> MHRFRVCALGAAFCVARRWRSGGGPGDRRVRTDWYRCYPSLMEEKDRDMYHCYYPYLFDHGDKMSLYPKIPDNPREWQVEQLQTTYDAIREDKYDAFVRLRAKFPELYQDTYAWDNPPPFGEFNMFYSVRFGMIGVKAFTCKDYDDLGNQFDCTAFWFPDNQIVKHSTRNGDVGTDKVYVGAMNVPVEFHKPHVAAFYKAAGVPVKHVSAGFPVTPDAYAPVGTKLDVRHFKPGQEVTITFQNTDYGYQGVMFRHGFDGGYVWLGDSKWQRRPGCMGAEGQKRIYPGHRMAGQTGASAETYDGVPVWRIDYKNSLIYLPTLIDADVGTYVKFRDTINTKGYTLWNEHRGTPPFPTFIPSEEEDLSKLATDEGQLTSPPLYMYFRDEFAAAQLVTQADVEDAKSAKPATAAPKKKVYDLKKYTEARKKYRKNLQKARKYKLMGVRTRAHEKQQEARRAKILKYKRVKT;> MLRLTQAVLRVQSHQKKRAQHPNAGTRFGRVYNRGFVRYGFGGFGMSVYSSKKDRTFKVMPVPPPPPATTAVEQRDDFADNRGLSATTRTLSPTFRMFALEDGGVLVSHPSHAQIMRWNQRVHTEEGKAANSTVMDEYVNSRIQAIIADNTIENTSLSQWRKAHMWNVIKSHGKLQRRWGTPDFVMGARSTLYNN;> MSRNGELCLQRIIVSYSPNKGNPAMRQFMATHLPEFHRQYPQVKIDIRPRQWPESSITGIYRDGSEKAYSIRFLSSMGINVRFHRLVNEGNDYNHSFSASHLHLQRRSVQGTWNPYLWNYEGTRARHKPPAQWSRKLTEKEWDYYVQQYGAQMKAEEDTIADRVRRYTDIPEASTEEVNQRWKEHVMPRLQTDLEYNLSHWKKQHRTGAGRPAPPTLNEYSLFSVPDHSSLGQDAIDMLRRREAQREEDWWRERKGQLKPPE;> MRYCRPSRPLVLARASSVLSSSRTFHSQHRTPIIPQVHVHDEPTAQRIHVGYYLHRHPVVKHSPHPLETEMGYLLEREQQRYSRHESAESATAFFASRGQTIDILGRTDPNQIKGNFFGLELYQDAMKVVMQRYTPEKRLTSADLWQPNALGDAPPPRHTLHRKLDDFLYLIVQEGATGKWTIPHTARKDDESLRMTADRAISSQNSEGLDCYVWSNAPQATVFLKDDNTRLFIYAATYLAGRPQFASFEPKPKDHAWVTRHELLQYSDTFKSAELLKALLDISADGTFEA;> MQPRRMAGHFNPTPQANSLAATHYAHTPELRHMADGAAMSLSGQRIPLLKPTLSKWSRQLRSDIYDELLKLPLRYALHDFRTLQAHIHAVPATATNASCTAAAGERLPPGVYHASSGLSSASPDAPAYYAVAGRDSAVGYAPPLGPADPVDVIPFFVHRSSNGHLPGKVYSMNAKTLMPAFYMRIQNIEGDMFRFEEELMKIFPTKKIFVRSHSVYVYNVNLDGRAVLHHWLLGLGF;> MTAPASHYTFANLKKLGLCAPQVALSRQPRLRPHVGHLNGLVYPLPYYAMWRGNHDKYTYNQATPARWGEGNTNTMYHQHYAHAKCPTDYGRGGREFQFLSVKRGKLKRKPLPTVQYVDPNSKPQWVFKSWHNPLSAPSMWEREVQYPEHTPAHTGAKRPLAVVAPKTSHKHLFLMHMEKVTVTVSPLLFGYGHTLQKAALDFYRRGLSARSPFPSDKMFLYYSIDHITPKIEVTWLDGSVYVPPLIEGVKAQDLIQMVMEQAWLAADRMSAEGRVLNPIAIDDYKWEQLIAFKQKRAKGAEAAKGGAKKK;> MLRRSPVPRRYRTAWRELLHPLPVWARRQQWLKRDTVEMNEAILREPYYRIKTFAQPAAFVSPRVSESAAHEPDTQQSSRYGVDRQLRGPRRAVSPERLQELREQLQFVGSIGPKVPPAAGAGTAYQDEYGTRLRPRYPQSWDTVPPHQPSRSEI;> MAFRGSSARLAATPGVGIAPETTPVKYVPEMLNIQNAKWWNGRGKPVYRSTYNEKSWLEKARWGAFTKGSRPVMRQRYSAAALKEALEMVPEGFETCDVPRPPQRIRAQSEGVVGRWYTNYWTLHSVRYQCQLAGVEWQFGERQRPRTNYDEPHMYTDFEETKAIRDYRSRWINVNRSLVGMSRRMKESEEEARYLHFKKVQDTFWSNRKVLVNRIKSMHNQGTLQSAKDLPIKTINIKAFLAE;> MHLHISSIPHRNSNNSKGGVLDATGPMLSAKRGALLLQAYHRPGEVISYKAGDYHLVPKKFTVGKRIAVRSYLDRNRTELSDRTFMPQKNWFRPYDLQDGCFDRDHERLSYRFYNLETKVIWKAFDTPELIGMLLHDETVKGNSGMYAPDMLDAALHYTREARYWRCIGITKPFYDRNTLRAHCWEDNGLQVGTLVMSQAMRHALMDLERAVRRKELGLEPNYLWDRWGPIGFIDGARADYLPRFEHNPYVDPDGVDVTEIDVLPFNTHEQIRERYRDFIEPDTAPFEEVFRSPSHGSLTTLADIPNASVVALYKDLKLKAGTPVAGDAVELAPADVRTLFYLSANPEWRAVADGKASWEEVVDAMQPVQAELDEKIDAARLLQNTRHNAERVRAFFEEKCGFHDFMYTPDKTITAAVLCYLTELRRICTETAWGAALAKCLTDMERVQGMGRDAFLVYRHIEDAILDKKRRLWAGRFAGESHEESTLDYLLENFGRRAERPRNVGTTGVEFDREQEPIGRQVQRRVLDSDKANKLAEIRRSRGKMWSKKRSVFDALHEKQLQNFNYGVH;> MPAYSEVKGTCGTPVLDQLIGYYVNIQSRKMYYKDFLRIEHQAVRWAFADIRKNSEALAHGLLQTGVRPGDRVLAIQPCNCETFVLQLSCAKIGALLCIVPQDTISADKLRFYLNEFQPRHLVAREWINVPEMKQGELVERNMHFWDTIYNVIPELGLSYPGQKFQWVHSQEFYYLKKIIITDHNMNLLGVTPMRKMLVWGPFSYYEQRLRRLSALLHPDDPVLALEDPNPAMEDKLHITYSHRNCVNAGFLFGQLMQLKAETRFGVMPNHHTDPIGAIIAPYAALTSGAVLVHIHSDMFTDDHAINGIEKLCVEEVETLVGRKADFDLILKHAGNFDADQFEHLRSVVIFEDGIEAPVSEEYLNKLSKALSLDDVYVFRGPIEASYMLTWRTLKKGSQGMVPHVEAKVVGDRGTSDAKVLVAGTRGNLRLKGPHVTAGYYNNAGLMTELIDEHGFASTSREAMIDGKDNITLMSAQTY;> MCTRVFDVSQRFILLVSLPPLSLSLRPSCCSRKAATRRRRSTASVLLATDALSLFVRTHYPSPLLFLLLPNFPLPIHSPRKQMRAAVGAVLQPSSSVGALRCQARFITRLYTSYFKGELFPNQLARPLERLPRGVSLAAARKGQQAAAPSSSGSGNPATTASLDVVTWGDVDSTDLVHANEQSRAVAPQAGLAPRRPYVPLGEVAKLELQGDYLTEGGLHQEALEYYGVVAKAYELAYPKDHPQVAGIRLKLAGAFRRTGRLTSSKANCEAVLQMLDSAVQPPLELIVEALFELGLTSEAMSDAAAGTVFEEAVALVDMFHNSGQSHKMLRLLPRLGRRFNLNFEEKFVYFSPFDYDRVFALADQCLERAEVFYQARNDRAGVMRVLQQRKELIDKKFFNMRDFAGRIHTMRGHWKRRAQVLTNAPTPDELLRYSPTIHQVYRDFKYELNAPIGREKEVQPGVNRVVHDMGNPYRRSGVRSQRMFRDAEKNFEKYIRADAFEA;> MPTTVLYHGDQLGPRPLVILDHSVARLEQSATAVLDACQEAAKRYEAMLSSLAWDHGAVFVPLQVSIGEINVMEQSCRHVCAVLDAMDVQWSHVLAHSYGALVAARMAASTAYPHRIGSLLLLDTPLVTEQLVRNTKQREEIAKAKKDVNVPPAELSFAIESLRSALETTLPYPAAVDKSLYEDHLFSSASVFREKGLVRDEHRYVPVRHLAQVHHPLQLLVPVKQPITDVAIHREFFGLRRPAVIKTADNHEDLFSAKCADEVADVVRAWMQRFEPDVVMKRRFEKAAKEMVQLMGSSASFGEKGGGNIEKSEKKEKRKGRQ;> MLSSAHRAAFARPTATLWASARSFGAGPTRLLLGLEQVQDVPTSTDRKPTGMHRGPGKRQTAPKEAAQYQFIKKWDLQMRETWDELEPFKGLPKPKVQFGNEAAEVIWPYALLLENVIKVHPYTKSIYVYYSQRQSTPLGELAARVAKRVSQAYLIPITFHNSHVYVEAEMLLEYSETPWVVVHCLDGTHKLIPVKPQAGQTVKEGAEEVLNGIVSACNEIGSAVKNPKEVMRLLSERPLQNQYVRVNYQWYGDTPEERMSHLVKWDYEPEEVVPQLRNRTQHVLDWMNYDGNLPTHNSVRVNIHREAARMRKPNVSAGPKTFFNSSGSRANARTARFDNSRSSQS;> MLRRTEIALKKGWTHNPGHTRRGGKNLAWRPKISDAKLSQFVPLALVHPRRHPNNWQERQFNALGYTKWPKDIGFYNAGDNFEVTPEAAWRLYVHARDEPYWGKLHCEKTIITLLPVVEKAPKENMERVLDVFRHYLKRYGADHYIYNAVMQAAAFAKNYEQAEQLFKEMETLGLEPNAQSYVNMMLAAKLCGLPPEKSEAYFKRAVKDGAMQSVMRMDTEFRMWMDQLDRLGSFTASSGYLSVNEEGAKPMPRDMWAIWGWHRSESKFISRRDLIMQQVRARVHSGKELVGTVYTKTRRQPWAKFNGMLRHDYNGPSYRAPTIFPDAPEYTNEAGHKAF;> MLQCTALVLKSQHKNVLRKGRPHMQKYKELNRWQREAQGITKWEQGHSHRPQPYVERFNPEGAGLTRGTSAYAWKWWHTQYPWLPNVAPADYVPPSPRGIRPAAWDDEFADVVLSMSDEEIQSYLLDKLTEVIFAETQRDGYELRRLDFEGKPLTELPERRIIENFVFEEETLRERVLDRVVEGVFRLVPTSTDRLELKSVANIIDFVLTHVTVARKPLQHEIPEAARTVMRSHPLQPQLGFVHALPTDNRDAVVQEWERMHHLDWQFGKAVYEPRSAENERGNLTWLREVRHHEAREAFQADVDSGEARRRHMAKIKAAAQVPHTGTTSQ;> MLRTTHVSWASTAKGYMNRVMVYAHRRRKARYLAPKNAHVRSPLAHKMPEEYGNTWDPRSGVEWHNRMRNRNHYRHWPWARWTDDPVRFHQDSVCHRTVSALSTVANNGAPEWDYYAEVGQAYETPSHFPLSYTAPFIYQYTAQCWSREDLQSYLERIEQSSGLRTIADAASRREALYTWWHNAGMNVIPLGVLQHLELVSRDIVAQNARKSYRIEQHERGILRTPEMERYYALPHLRGPSMPVQLAQPSGKYPSGKFTQMMEDVAIHPLQKPDARYKHNMYPA;> MQRCLARLFQAGVHTPHGSRYNAARMKNWPVQEVPQNFNFTNEQRFKAKAVPRDTGKIPRDFLLSVLYRNQPCEVASLWEHCLHDPQIVLDSKRHLREVLQQARAEGFVSFEKDAVTDRWVCHLTRERFEEVRALVGARAEAQDLYSGLRGASATETSAYSESFREMNEDTKREHFRLLSEQVADTTTHLRKFQRMEMDYLPYTDLNGKVNFMWWYEMSDTRDATALPEAAAEGSPKLSE;> MLYGGSRVQYLVQPPFTLHKIRSENLPPPSLYAERHDLGLEMQLPRDMHVYNSINMAIQRQVGGDSSTLDGEQQQLQGGHADGFDMGAFFTEQHHPERHHNSSLPYAKHDTNNVLAMRLFPVNVGVRARTEAIRIRTDDCLQRLRDADLCAKMRLPLEHPLPLSRRSQYAAIHRVRQERCYDAPTEAAGERAAAAAEEASRTAHLRGAAAHPPPSELSIVTRPVDRLGSHSGSSAAACTADADHLSFPVHPFAAAAVSSGCHSARSGSAARLASQRWLPLQTLKPMGHNWSAATRSSGVRGPHMQLMQERLDQKGFGWKRKSRSLWQQDVATAGFRPHRYF;> MLRWSRLLREMAPELQLEYIPIIFTRTILGPQGGFAGEERLIKREVAQKYMSEGNAVTPSAEFHQGVWCYNPDSEQYDRFVERNAEFLDFAARKRQWLDVYWRVNTGYLLFGRQSWGQGWLLNCPLRKKDIAQKLWEQYKVRVDPRLIEFREKDRRTGIQDLGHNWCWLYLPGAEELAIDREVYDNKRVKVRMHIRKMSSYGALY;> MRRLPLFCRRPSRCCGATASGSGSSSAAVLAASAAPSVLVLAARGIATSGRVTNEDRRWWLVHLECAPDVTPGTFVSWLDCCGTHTTKKLIERNIWTIEQVAELDSDRVDELKYKEGCLKMDVVWEHARTIITPLKQREVSGGVESQLQSRILELRKKRELERQRELLARERATVSDKREETLRRLRESVAAKKAALRKKLDEQHGEATPAASESASTEAHRGTAEAAVEDEAVGNIVDRMSGGNPPRA;> MRPSALCLGGFTMKYKRGTGLWDEDHVNDFDANKYLSARSTMRWYYGMERLQTRNNMNARRATQSYNNNMGLHHSGRGAFERELERRGIQVDKYPLTTTTGAARVAEMVLLRRQELEAHAKKAMESQRQARRRDAPSEWYDETEGPLNPRFLASMQSNYTQVITELPSSPVTGRRELPGASFA;> MMLQHTSLLCRKALQSYPVPPRARNYERRWSSSRTNPYNRMFWRTVLNEDFARPSFWVSDFRHKYLAKHGMDYQGRVPASPAPGMYQGFSDVHKILANHPKPQRESRHLPVMPMTPRVVFEHAQEKRIDYAKKMHRDRRLVEQLRTHEFWGWYMKLQRVRGRWCKEHGVSSRGVYGPAVDAAELWG;> MFQRTCTPRLLACTSALLKRSGKPSDLPDYKQVYLPYDTAPTKTELDRERRKFMHAYSGRMEHRKMVEVKDVPQNMYTYGKEGMSIPISIFKDQADPVIGPEWTYPGIFENKIVAQHWYMEELFDREKSNTFESPWQRQVLDNQVKRRLGKVAWRMSMLNIKTIDIFHKERGASKRPGAGDTKAPATPAGKK;> MSSGAVGRGSFHSVVAGANPRRIPTYYNSAYELIQLHRAHREVTRNFLVRDKVFDNKFPGCSLANGLFKMVPNKRGNFHTRELTESIRHRTIWGQRIQQQRTINAAILEDATKVLSPAQMEDRFSYRTPDAAAYFSPQEYTAANNWPNYWQHPTEKHVVPKPRWRREPELGGITRVRDAVATPIADY;> MYFYRRIPSLASKMNHMRQFSLPRSSAAIIMAASTAALAVPCRAMHGKPASGHKVRTQHSRRWWMQSKAHHLTAVPHEEARSRPHFPAYTEDVDQPMVVPDGVCCFNCDKPIDGDDINSYVWVPSGNARVPTTQGYFFHVKCFKCWNCKYRIIHNQFYSKDSRAWCLSCALGRDIRVPTRRWHTSYVNTHRTGSRLTGQFFPRHRHQMEFLFSPKE;> MLRIGRTLLAEVTTINSTTASVSGRLIRIRKKSKWIDRRSTRVPHNGKDIWYFGDQPSCALCHIRFRYKQDYEAHKESELHVNRLRWVETMNWWRETGEPAYLKASNEQWEWFEQHVLPTKAQEMGCTLDEARRVYRQAIMTETPTWHRPLQCPTVKQEVQEPRDQRWPASPKW;> MLRFTQVIRKNPVVFKQGQGMFSHQLKRILNKKSLHKYNWDPLHMYDPRKLVHANRYVDHDTYEEKYDPHWEHNAHLVPDQQFYNIPVPKEYKDAYWWRDLQARRVQCPTEWVHFRMHTKDKLKYDFQDLAFRKKFEYSYEDVVANAKDMCS;> MYDSRSSGVHDVAPRDGVDFMYEGPQQVLPGAHPLPLFHPDNSVTRPPVSPYLPSPQRPHPYFTTELPELPHFQTTRPIVYTVGTMKQRIVAPVFDLANNVTHTRELDPFIFGFYPETEEMAKNLSYWLVRCQNFSSKWDYENREIWRKAKKNWPNTGMGMARVGDRKNHAHPWGAHSKPVKPWNLLMPTMDVKTWSKSNRMLVTLKMLQGKLQIVERLTLPEPTQEAYLQLCRTMGWDVRHKGGGALFMDGGSRLTPSSEYDRAFFFGSFFNGRNKLVRPTLLCDEPYDYNRTSSKARTKGPKGQKNPIPINRFNAYDALTHDTLIITEGALLQLEDEMYTHKLAMLPPHIRAQLPERGFLDSEVLGDVPPALQTVQMEAAARTEEAEQAMYAPYYDNPYHPWQDEGEASYAVDAVEGTVQRYIKSRKTSWAMLS;> MAQWIPKTAWKVSNLNKRYGAPYVAKGYASLDPRCSLDAYSSFQQTVTSADMKKALLSIDSTSSGALVIDVRSEPERRLRPLLSPAIVALHPHDILSGAACPILPSNKERAEMFVVASEAQRAVNACTALRRWGFSRVTAVSVDAVSEAIAAVQKPADAATSSSTKS;> MLHRSCVLVDSFKEHYHRVHLPRRLALQRYIKREEARLSRHKGKAVAAAAAAGVQPGEVAYKYNRWWVSNDHEFVHQFAFVEDPDVTREKRNTLPLVTKENIWKEPQQTFFLPFAPFVRVVDYAKDPDTKFLKPVNIPRWKDYMQRTKPIVPRTWY;> MNDIYARRLAQTSMFHQLMRSHGTLWAATQVTKEKLNLAFVKEEMMRVNGRRAMPLLIGAAANENLNDTHFTHLTEHCAWTESARAFAVQRQTPLTQHIASMGRMAETITQAKTASTSQLLFNEHLARIDGISEFEEEPFVDDEDDS;> MSNRFFQKFYLRCGNCSAIQRSAQGYQPIANPILFKSDEHCRNYHDEQRRAAGYSGMVVTCRCHRCERVHSNWKVLDAQQFLDAKLRMTPEERAQRLWVSKS;> MLGGLRPLAAATRRTVGGALVSPALITPSRALSVRTEDFFSKEAVSHARRVSWAPHTTEKKVGAFAKLSRSNFNDPLPVSFQSEPYFEEEIEAYRAHHRPDVYVYKYNVSPTHLSLRE;> MRRTVRALYNSFERGWKDKTVHPLDRRGRFNLDEAAAELQLDEAYVASLYKPLHYTYSMKGQRYPAEQGRTSRPGSLAASRDRMFPLYRRNYKLNRELRVLDHRRISTD;> MLARYLDPSVHPLRVGQVVAYDYLHAAKTWQWTLGTVREIKDYTAVVQQWGLHTGDIDTLRSILLKEVDTENGRMKNYHDMLAIAREKLASIRRSNEDRVSHVRGHFDKAREKVELIDEVDLRKVTAQAAPSPVAVAVLKAVWAVAKCDPTAVEFYEWADVQLEYRKPAALDEIAKTDVLAKLYPSAESLQQSLEQDPKLNYKAAARDSPVVASLHAWVITALAYQQAYNLLAHDKRIQEQNDAIAAAIAGMKACRAKIAKLKDELSSKDTAALPGQVTSFTRTSVLVTIPLSAVISPVNVDTDVKRCVLTKDEVEQIPIDAKITRYAQKQKLAITGSHLLDQYAAATTTHIYVTELEDRLFFFQHYMASALRDAQTAAVDAHQRLAVSLHELEAFRQKRHDAKKARAAEPELADADGVEPSSGPTSSRSPTGRAAPRGQSAAPRGTASQQHKLLGPAYQSIDPATIANEPLYAVTIEEYKAKDAAGERAMDEAERMADEVQRLAVELEDAKAAADKLAEELAAKDEELAAHRQKRHDAQQARASDPALAAADAVAPRSGKGAASPHVGAVQRQAVDPATVPVAPAVIAEEPLYVATAEELQHVRDFADQLAEELEAFRQKRHDAKKARAAEPELADADGVEPSSGPTSSRSPTGRAAPRGQSAAPRGTASQQHKLLGPAYQSIDPATIANEPLYAVTIEEYKAKDAAGERAMDEAERMADEVQRLAVELEDAKAAADKLAEELAAKDEELAAHRQKRHDAQQARASDPALAAADAVAPRSGKGAASPHVGAVQRQAVDPATVPVAPAVIAEEPLYVATAEELQHVRDFADQLAEELEAFRQKRHDAKKARAAEPELADADGVEPSSGPTSSRSPTGRAAPRGQSAAPRGTASQQHKLLGPAYQSIDPATIANEPLYAVTIEEYKAKDAAGERAMDEAERMADEVQRLAVELEDAKAAADKLAEELAAKDEELAAHRQKRHDAQQARASDPALAAADAVAPRSGKGAASPHVGAVQRQAVDPATVPVAPAVIAEEPLYVATAEELQHVRDFADQAAHDAATREAEVAGTVENLRNELDDVREMNAKLEDEVFALKEQLSDAEDAYKKLAGALVVAEDERQELCDDLEAALDELEQKKDEYDELLGNLEEVQGLLEAADVAGRTAVEALEQRNRDMADLQGELANALDASKENENLRALLDAKEREIDRLKEYNSFWTDTVGTGKQKVTHRLTKIFDGDWTRLMRHRPEALKAAFVIDSSNACHVPGDQIFLVSNSFTRRLLTRTDHCPKCDRLSTFRFMSVSGMVGRMPYKPVDTPGPSYATLYWRKQRSGKIASQPLNEVCNKNEF;> MWRLSRVALQSNRAALYMPYTPVATNPVVYFDITAEGDALGRVSVELFRDVVPRTSENFRSLCTGERGYGQCLLYYKGTPFHRIIPGFVMQGGDILTKDGRSNVSVFGYPFPDESFEGKAGKHLPGTVGMAHSGPNQNGSQFFFNLGRNEQLDRKFVVVGQVLGGWEIVNQVVKLCGSRCGTPVSRAWISDCGQSGGYMAEETQEALQGERAQHVIPGKEVLDLIQPRY;> MRVWVLAPHSLPPASFRPIFEARPPSSPTHSFHLLPTPIYLYITCTDAVDLYVCAVTSLLAEWTTTMFARSTIRWAAGAGHAFMDIAIGSQPPHRVTFELFTKRCPIASENFLKLCTGENVLPQVSSIDGIGEPSFRDQFLPQLTYRNTTVHRVCKGYLVQGGDIVSGQGTGQLSIYGESFDAPEEVKASKFDRMGLLGTAVSAPHLNGSQFFILTADKAPHLNGTCICFGRVVDGWTVVKAIEAIPLTAAGEPAERVVVVECGKL;> MASVSPLLMPCRGVKLVNPIGKQGSQHYGLEPKLEAGRDTQLKHTEMYDGYTDDFGVFKEGPPVTLRLEYVRSPDHGYSQHILQKDIWSPFQVGANMMSYTPLYYDWKGFSSRDYFGHRSGTNPGSKVLLGHYRRDEVRSWGYRIMVNHKPQKRIPKWLACVVHIPRKKTFLGFFLYANGAYVAELLTYKQLPRIIYNKAFQGCLPTIGQTVSLTEVTYGKEIHSVEMYPGHGGVICRASGTAAVVLRGSEPNLVPLLLPSKEVRLFDNMCHAVFGRRAGVMYNKQRNFSKRSVEENMPHRPKVHSKTKRVSSHPAGGGNGGSPNLLTPLDWRIHPRNCVKTKYWLSGYILRGRQYNRNQTVADLKSKTYSWANRDPVYR;> MSVFPGLCGDVATTNYRVFLGTLPNLAVEERFLRQVQPVFPWYASRKHVKEQASEFLEIDLASCDPELLLRYTHVYYVRRQLYDELVDRQLTLMETGKAAKVADSALLTCLAQVNAAITPRLQYELHLLQQAKKACRVPRRRELNPDAALEAHDYLCMMRVVEEDVGGIPDAEMQARAYLPREVLEAKVKELAAMIFGDGGSATKGTGAALERKEQKLLQRMIPADYNKVGAVEKLRPVDVTALYRFTGERVCGRPADKPFARALWGHVFRKVGSHPLYLQRASLYWARHSGLDPQSATSAMPADLATAVCVQQALFPALKYRCQYLYTSPDIARQQWRTGHVVPLLRLFPLLGAPAAEDLAAQLVVEGEWAKLGIEADTNLLHDTVLRQLKDMVEQVSALYESDAGAVLKRVEDGAKVLCPSLSERESLTMRGAPEDTSREVSAAAAARVANAAPA;> MLRFFRARLAPTTTDAAAKLPAGNPVNKTWFRHNLIIRRKGSYRSRWGNGTEGYGAGVPLSDQVKLHCVDNTNCKHVRLIAKATAERFAHCRVFPAVAHRVSVQRFKGRGGGGEVSRHRVKPGNIYWVCLFTRRQTNTRMSGLQTNFDRNTCIIMNDQRVPLGTRVMYCAGRHVNHKYHLKAVVLANFFV;> MRRRDWCGVCLPAATLHALARRYSEYRSSYTGARSAPWAAPEAAPAYPSARSPFPLERPRFRKTHIEWMLHHGHGDRYGKYGPSREIADFEYADGTPSSISGKRFALKHHQDHLLVQLIRSAAIVERFEEEELLPRIPGTPEQRSWDPEIPLFLEDVDEFGRPPRPVAGNMVARVIEERFAQESGRTPVNLANKHAGEVLEPNTMFATYDPAAFVSDDIKKDVRRPFWSRRRWALSDNFMVPMSPKPKNTIKDE;> MVLNKWAAVTKSAPPAAGLRPLARTVSPNPKLRPADYKVPYVLRTFIKDRHSSEMQHIENRGMYREELAIERSRFPRMQKTLTIQTDGSLNEREFEFAVPPVVMLFQDRLSAHRQRQVALAKIGKLKRVKSWETSVRGKESLNPVCNALVFPYCVPKKMLVRPRIVDPLSAKSMADNRRSRDDPS;> MRRSAWVFVAPWVPPPRHDVKVTMPPPPGGEVGGSYGVSTGYSDRLARTPYWKRMALSTYALRMKENETRYPMSPHREGEYDLRYTVTAYPDHIKHRPLLEIGEAHQIPTIEIPVIFLVNLWDEERLTWFGRQYETVYVNRNVAREELLPQRYAIYATEEAYKLLGLPVVNHSIHEEIPKTPHAYKKLLEKQSYTEERWKYTIEYLFRKYEADPPELQDKSEDGWDGVEELATSATAGGAGDSLAKRKGPVKQRKARKIKLF;> MFSRGAAATAMAKVSRLVSPRLRIIHRDYLTRRGGRTHQRCSAVAVDYTPTYFATYKSDPGQCPRLIDAEAVHGDEQAFWSARRDFYRGGASRSYYPAWDRQAQALIMLTREVPRIPQEAAFRLFTLGLKMMLLPRLVAGVELMLPSWVTMNAESVLNEGLEGKVAEADGDGKATGAAADAAALPSASSAGANEDSGSANAEKR;> MLRRSAVRYLKARPKTVNIEPGSNRFLDPNVEAKAKDIFAVPEFPNKAVLHNWRFFIKAGKAATGPPVGQEFSKLGLKAMDFAKAFNDRTKPHFKDDIELIVRIQVYFDKSYIFRIEPPPTAWFLLRAIRKKRGETGPVVLRGNYCAYLTLEMCYEIAKMKQMSWGKVEYPPIEVRVRRVVGQARRMGIAIIGIDTVHSSPVKGMTEKQYLEESEKHRKVHMIQYEALKAKELESAPLIERLHRPNMAPLTNTQLEEGLKDANLLNALWKSSHPKSLFTQDTRDREMARRYLNTRGWFKEMTPEEMRVVFLNYRLPKQEDHQRQLNMTNGQAQSQAYWSRDAASPQ;> MSKQWLCREGERWWLLDARGQQLPHVAKIAAQYMTGQHRPDFTPGMMTGDHVVITNIKDAVMTGDNWIRVPITWQTAYPGGKYRVRLSEMYERDPCMVMWWYLKDEVNRHFVRKLKTRTAPLEKAWLYEDSVHPHAEKNPRPLVWTDTATMGWRYKDPTFQRRWSPNQFMS;> MLSISAVQRRYRLFHPVHQTVPFHFNPVQSIFPLIYENNLLAKPRLSWKDYEGRKEFDADHPLPVVGTRLNERTTTHKWSHWDQYINPQITQSWMYLTQTPEYVGPRSGHNVIKMGWMKIGGSWKYSRSYNDARRGFAKGQWQERKMTPRFMLAPRVSAGGPRNRYEGKASFSRLSLSKLLWAVDTGRLNPNETITLYHLRNAKVIADREVVWPGMVLLAGNVERVPYPLHIELQNASAKAIQLLEEAGGSFTNVYMSHEGLYQELHPEEFPTFMEQELPERKGLENFATNSRKRGWLAQWYEDESRYAHPGAGRRTAHYIRPPTDRDFPATIEEYELAKHHQKWHLNQPGSATVLPWHSLNTADMARRSAGRL;> MQSSALRPSSLLRAYHYVHPKTGRPIRQYRKYGDPRFINNEVALIKGLFALITTDFGMVTQSQLENARLAILRRMPRGSFALTMHTDYEEFPVVQKSPESRMGAGKSNIHHFAYKFTTGVPLFEITALSSRRLNQAEAEGIFLAGRSFIPLQTAVVPRGRVDEYHVFK;> MLRWSRLLRGRPPPVMGHAKRMRFAGVDDNPSVTHKPWDTSEPLMADYGWERGKLPKFRARSPFHRQQIARRMVTELIRKDYVIVGGARAPALRILADHVVELAKAGDTDSRQQLAYFLHDPLMVDKAFDEYPRRFRDMNAKYAMMTRLKGRRRSDNVAMYFVEYKNRDMSDNHKGEDYTAGPERFFLPPRIIETEKGIQRPPHMQMAFDRWASKFKTEEFHHWWRLRHAKLRYWGVRNVPHPSDVDPLWTEKEEEEWHNEMLANTSDFEDFDLDDDSYEAAGEGGSQGGSSSLSGIGPEPQKKY;> MGYTRERTNRHFFVSRANAFFSRLPISRIQRALAMEAIKKGSMKPWKHTKEQIIGSPITCNFEYNPRPVRLIGTVMDAHTEETSIKGGLKVYARSEEANMMLWIPAGNPKLKYEVTAAKGSFEHYLDERSKWDEAWLTGRARMK;> MLRSTGVSLYYRATAELDRLRGMLRGRARLERKVGLKRITFLMRTQTRYRVEQKAHWERAIVRKNVDSAAHEHGSGWQHLRNDLARQNLMLLPRTQQQLAQYEPLAFRAVMELCASRVAPPPPPMTAQVPEEAYATRPEDPKVAHPAARRQLEECVERMLCTGRSDVLQREGPRTTQAWMDAWKEYDLGSAAQK;> MLRSANPTIAKALQPLIEGPKFAVVYCGNHQYKVSPGDVIAVQRLRAPIGSQIALKKVLMVGGPRFTAIGRPLLEHVRVTADVEEQKRMRNVVSLFSTPGRRRLRWLDAQHAATILRIREVVYEPTVVGELDKYDGVLLKDFHADRHPNPVFTANDGYDLYYPKDWNKVEEASAFLEMMEAPPTEK;> MPKPAPRYNIGLRPAPKRQNVGGQFLATQKHYARELWYKRQYYSTRPFAIQKHMGSTPRILLDRTLWRSCWLTKSNLPDVNRWEKVVNSQRVTEDRWALVEEDGVMYQVNWKMYCERLETELQKAQDQLPQYSFMMKAVPSAWKKLDIELSVLRGLSVREAMAQCKLSPRKGHMAVFRALEVAQQGAEGKGLDKEHLRIAYITCMPGPTDKQVDIRSRGYYAWKTKKSSHLLLTLAEDPEMVLPDRTAIPYASLMTMKRAGLRTEPTMLDVPAITAEGI;> MKRLSSHHAIVCGAASATAASTRFGDVVGGGSSCTATSPLFAAQRGRFYRPLVNQGINLWRSRMGRLHKGWTTWEYNRDVIPDPRPFPEPAVNNYFGRSRIWNPIAGKIGLVNRKAEEWGWPHQRPPPTGLRRSPEYFPFFFSRYFPDVEVRLVLDSVLNNETTRPIFHIPQDMSKQELVNYLKNIYNIDNVVRIRVRNMRGRRFKNEVGEIKSLPDYKVAVVELDSPVSIVFKQIKGTEDTPDNKPAAQIT;> MGCVRVRTGCRIRCVRASFTYTQAQMYARYRTRSRFYKRPEKMLKAYNVSPNLLRLPKVKPGLLKGIYTDEKIDLRDRERLELVESIRHPKERDFYQDHTYHNQWIARDLESHQKIQIAGRYPYFSPDYEIKPWIWYPGDTVEVVSGEGAGQRGAIIAVVKYKNEILVQNVNVQDVVIPASETRPEQVVQREHPISVLRVRHVDPSTNQLCHLEIVKVRNKETGELEERRISLESGALLPIPAPEETVEAGDPLKDTAIQDADEETYDREKEMPLLVVRRLQAMENYFVDSLQKSHEYHKALQMRNAQDMQTFQKDVLVRATEKLAAAAAVAGHGAMAEAGSQAASVATESSQAGDAEEDAVKGTITVETVVAEVLKSEQRFRSDAAAPGVPGWWQNMIDAYVSVLEEEEATIEAEAAAQAQAAEADRRAEQLMADATAEAGQSMEEDGTMEGGDEDLDEQDGDLDEDASRSDRSK;> MLRITPSRYASKVTAGNAKNQAGSPRQKAKLFHVIPGTPVTPVEKLKEQRRRFGQDRYSRQPEYRPGRNVRMDPNTFTLYATTKGVMTIRTSRINPSYKWLDVEPDIQKVYRSRCMRAALQARGKASMMVAGNVHYRAELDHVTEPHWRERVMRVPKATERFQDPNYFTRGLVPSLRPLSRYSYE;> MLRQSSLLCFSTFALNPETSRAPHGPPRGLINRYISMGLPPWAAWCNRVNRHALYRMSDVSPRSFLPKAPHEMDVIWMNERVRERVRTSRQVQHVYRQLKYPFVKTGIHYSDTLDHWVQVPMVEAAMFEIEKDGGFDNFILKRSGPELRSTYGERIRRHLLVRQKETQKNFVLDQQAKALAEVTQAELMKATSEEELDAVLAKYGMDAEEFKRLMAKRVMEQRKSVAAAGLRSK;> MRCSARRANVAALYEFVDGNFLNNKRPAIPGGAWPLESLRRKSLADLQQIWLSLLKERNMLSTIKEHYLRHQEELGAMPAPSRLKMVEESMENVKRVVKERDAEATAEAVRIFKERLAKGIYRYPPGPPPPPGAHDPTSTVKLVLSRRVDEERLRELLGRFNVFEAHKGIVKLTMQLPEDVLTQKRDAEQLWQQYMAERRNVEEYYKWPGSSTGSAESASVYDHTVVELAPGVYSGHRGTSAIESNCVDDSNDGAHGVVQAARLPVPPPKTRPPPPRNPLEHIKYQQRSVLSKAVIQLGYFPNITTTAPRFTKADDVPRPVHPDEIEGPWEVRVTYDAKDGLAYVQSLSLTSIDGAAVLSVEEEFPAAAQPYAAVDPVYQEAVRREMAQEETLMKWPNVPKWKYQYDLYTKKHLAQVVQYNYSNVVDYVDREVLLTGRSVWESPIDIDPTCGGMKSVPAHAKKPKRYMTHGLAEVGVTDI;> MRRCVMAKGEDPAHVAGWDDRQDAVEWWWTEANDSRGRQRLEAAAAVAAAAASSTVGLPLFPRFSPGRRRRRRPPAPPPPPPPLFLSRHLHSMPWLWCTCVKMQMYYTPTALTCPLSNSLAAHVGHIIVGVAALLPYSMLLFLTVMCNPRKHEPVLRAQRIRWLTFHSLMFRLLRCITASPAVAASVAVAAAQTPTSLRPAAVCRRGVHLAPSVLAASAPPPPPQQQQQPTSAAVPASTATSTTTIAAGPYRRVGNVFIVTCIDHPFKFSWEVNRMLRELRLEFMGQTTVVPDIPPVRKRIWRVRHVVRVDQLDLDEAKALIGIPEHISFRDLAGQIPPTFGRGGSVANPHMRSKMNFMRLRRMRLRDVMHRDQLEKRLLEERHHALQQQQQQQQGGGEAAAAAAATTA;> MLQRTTLRCYSALVGQATPVLLGSKGGTPKRKKNPMQLRRKTYGLHFKERYLKLEEWYFCPLCAEPKKQGEWCRREDCRQIKP;> MFRASCTLLGHGQYKTRLKKRMVGFIPKVIPRKIRNNMVALRSEANTGHMEGYIKTEAERLDATGRKLQKTMWDPVLQRYTLMKETKVRGPFLTKSNIARKVDFPVGALHGTKLGGKK;> MFRISLICFPKAGCEEITRQGRRVVLKPQEYFAQHRMQVWQMRFKEMGPPFSRVWVALGGKMRRRRIGRQIDVKDMRYYWRPIEPQYQRLYMSRLRIKDHSNKRVQPMRLRATNNDIGQASSLKEWERSSDRKYGAALAPPKKRDFEFRVF;> MLQYTSSARQALRATALVLNFFPLGYTCGPKNKQVFFPPNNLDGRTTHQMKKLQGSTDKHPGLVPRDKLKLHCEFCRFHWVQDTLVVRCAAHPKEHNQREIWLEPTWTWGKQQPYQYYKYMPVNINPRTGMPLAREDAKGMNNERRSQGLPTKTRLLERERRGISRAITGLGIYNQRWQTRFPFAT;> MRRFLPSSVAAWGAGRVLQCAAEWYHMPGWKTQSSTKDARSREQRERDRKARQIEKLPRPEALHDFQYPYEKTILSDSMFEYPVYETELDTPQLFNLTPPPDFFIYWNATDFDRTAYPPVPEDDHRVLVPSSQSPRWIEHRARLLQYLRKHEIMPHYVPHIHANVNLSVVFPGQYNTRARLTDENGDKIPPPPAQTKMTPRNFWFTAHCGNYMELTDVQQPPSVFFFEEAPAAASAASDAGEAGDAANKQSSHAAVNYYTFVMLSPDYPYRVPLLQDRHKADRGFFLNYMVANLRAPQAVSTVDGAVVDTEGLQSKGDVVVPYVAPLPTEDAGTTRHLCLLFKQTGHVPSVKPMTATEEQRDFPLAQRSNYRLHSALTKQTGLKMPPSASTACLASLRSVERAIPADPCAVSFFTTKWDIQVQEYYEKVGLPEPAAPVDEEIEALLEFHAMRPEKLRVRARHRPDGSVNMGDDPNFWAQALPTRAMDGSMQRGLGWSRRTTMGANGVPVVYPH;> MWTLSRPCLAAVRTAVLCQKKQTAAGYMASAGKVGNEEKWAQAAMEYIHEKNHVNDARKRQQDVDQERSIANAYDRYSAVSEAKFDERLSRLIARMSEALEEMRNLGLEEALEEAVLLNSEQPPGHYRRPSLTPPLAGYEPGFGLDVPQLRSQQAEYPPLRRPTDWLEFGEGGADDFPYVDTHKIEDLTAKHEAQLEEQHGVLREAAPLTGVEGEGWEAYVALHRKALARQHLIMDLHNDPELRDKYNADEAFRAAEWERRGMGALSIEAPLERDLELHYAQVPAYEAFRSH;> MLWCTGPRRI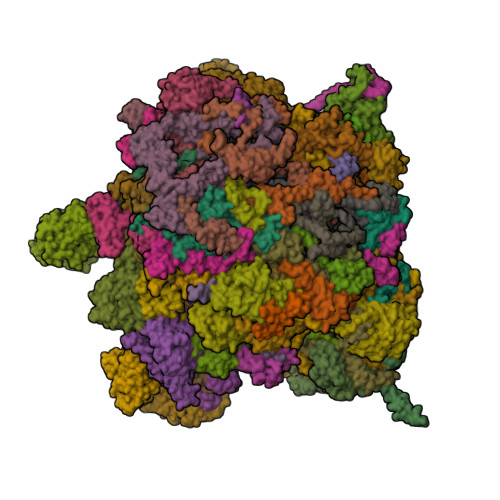VFHNAPSVYPFTKPFHDTPYDQDRGRFDKTKNILRENKWPAWMDHGADGTGFGIGLNRTHPLSKLRGNLRRNPSEIPRVLNMMIQGVWHKSGNKLYFRGGKPPNPSTHPYLTGEPCPVYGWKVTDPGVIREFNLPQPEDKTRYKPYVALQERKIMGMQAPTKEHSAASTSAASTDSKPLMKRLFFWK>[4x]DKPVAHVVANPQAEGQLQWLNRRANALLANGVELRDNQLVVPSEGLYLIYSQVLFKGQGCPSTHVLLTHTISRIAVSYQTKVNLLSAIKSPCQ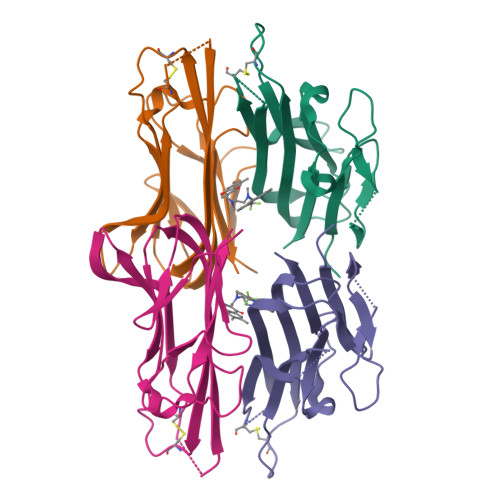RETPEGAEAKPWYEPIYLGGVFQLEKGDRLSAEINRPDYLDFAESGQVYFGIIAL>XRMKQIEDKIEEIESKQKKIENEIARIKKLLQLTVWGIKQLQARILX[6x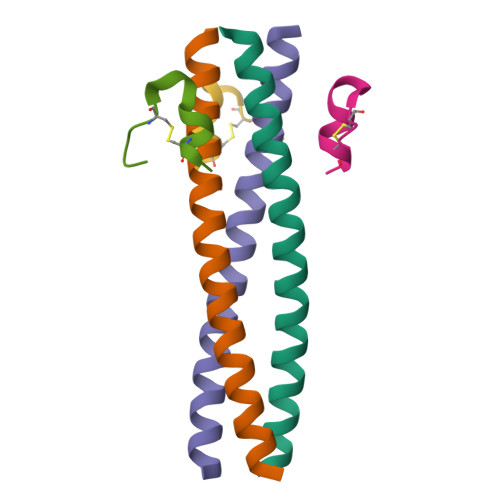];>XKGFVCPPEWRWLCDLX[6x]>[2x]GSDDKVRQKEMRKGIDLATTLERIE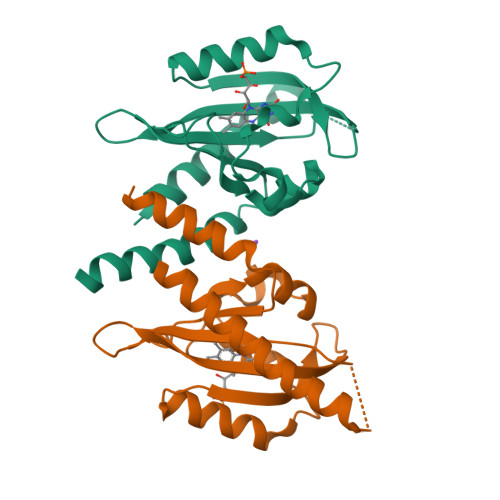KNFVITDPRLPDNPIIFASDSFLELTEYSREEILGRNCRFLQGPETDLTTVKKIRNAIDNQTEVTVQLINYTKSGKKFWNIFHLQPMRDQKGEVQYFIGVQLDGSKHVEPVRNVIEETAVKEGEDLVKKTAVNIDEAVREL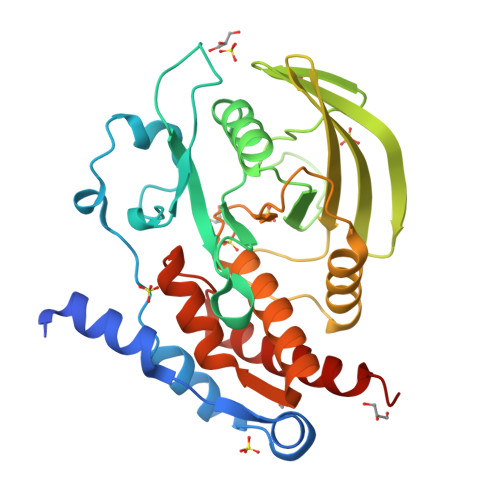> MGSDKIHHHHHHNTPREVTLHFLRTAGHPLTRWALQRQPPDPKQLEEEFLKIPSNFVSPEDLDIPGHASKDRYKTILPNPQSRVCLGRAQSQEDGDYINANYIRGYDGKEKVYIATQGPMPNTVSDFWEMVWQEEVSLIVMLTQLREGKEKCVHYWPTEEETYGPFQIRIQDMKECPEYTVRQLTIQYQEERRSVKHILFSAWPDHQTPESAGPLLRLVAEVEESPETAAHPGPIVVHCSAGIGRTGCFIATRIGCQQLKARGEVDILGIVCQLRLDRGGMIQTAEQYQFLHHTLALYAGQLPEEPSP> SGRGKG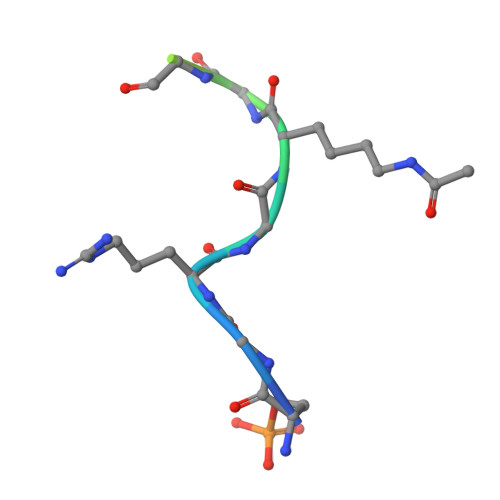GKGLGKGGA(2R,3R,4R,5R,6S)-5-acetamido-6-[(2S)-2,3-bis(oxidanyl)propyl]-2,3-bis(fluoranyl)-4-oxidanyl-oxane-2-carboxylic 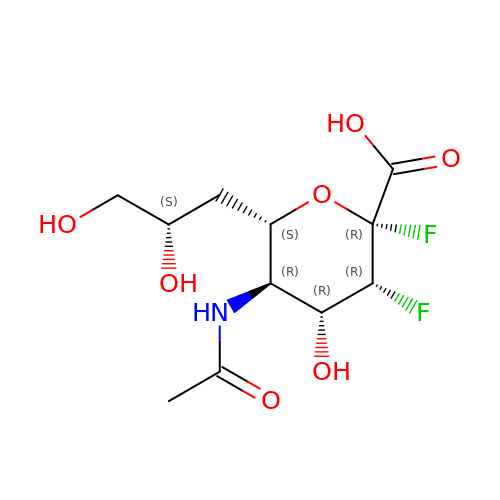acid | C11 H17 F2 N O7 | NDXUMNONGSWWQV-QYKRXNJRSA-N> AMALTGCSEKININEDKISHKIDIPDSAWTIGIGEKFKNAGHPNVKYPMIDDSYVQGAPLGGFGAGTIGRTYNGGFSRWHLEIGKNKYTTVYANQFSVFQKVEGNKDGVAQVLYAGEPENGYLSSWKWDYPKESGMYYALYPNSWYTYTNKDLPVQLAVKQFSPIIPYNYKETSYPVAVFKWTAYNPTNKNVDVSIMFTWQNMIGFFGKQVNVNSGNFNKIIKDKSKDSEIVAAVMGNISNDNEEWNGEYSIGVKKVPGVDISYKAKFVTTGDGSDLWHEFSKNGILDNKDDETPTKQDGIGSAIAVNFKLQPGQTIEVPFALSWDLPIMKFGGGDKWYKMYTKYFGKNGKNSFAILKEALNNYQKWEKMIDDWQKPILSNKSKPDWYKTALFNELYYLADGGTAWENGKVGEKDKRTNNMFGLLECFDYNYYETLDVRFYGSFPLVMLWPDIEKQVMRQFADTINVQDSSEFKVGSNGAMAVKKVQGMIPHDLGSSYALPWIKINAYDWQNPNIWKDLNSKYVLLVYRDYVLTGKTDKEFLKYTWKSVKTALDKLKEMDKDNDGIPDNEGIPDQTYDTWSMKGTSAYCGSLWLAALKAAQEIGKVLKDNEAYIKYNEWYKIAQQNFEKELWNGEYYNFDTESDHKDSIMADQLAGQWYADILRLGDILPKDHVQKALKKIYEFNVMKFENGKMGAVNGMRPDGIVDESDIQAQEVWTGVTYALASFMKYRGMTEEAYNTAYGVYKMTYDKSGKGYWFRTPEAWTKDGNYRAS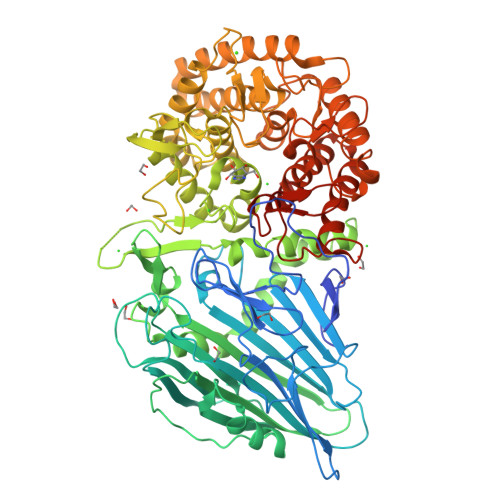MYMRPLSIWSMEVNYNEVLEHHHHHH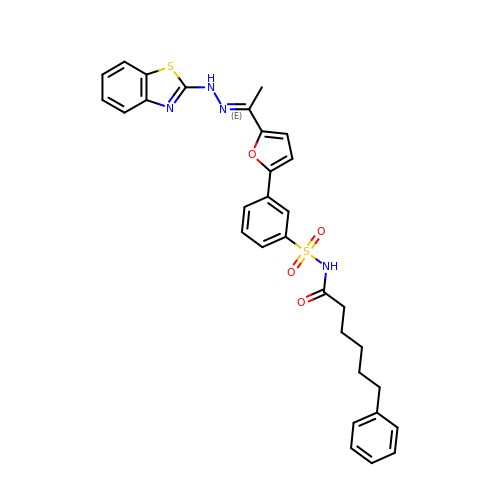N-(3-(5-(1-(2-(benzo[d]thiazol-2-yl)hydrazono)ethyl)furan-2-yl)phenylsulfonyl)-6-phenylhexanamide | C31 H30 N4 O4 S2 | ZGVBPNIFKPDHBC-STKMKYKTSA-N> SRSKK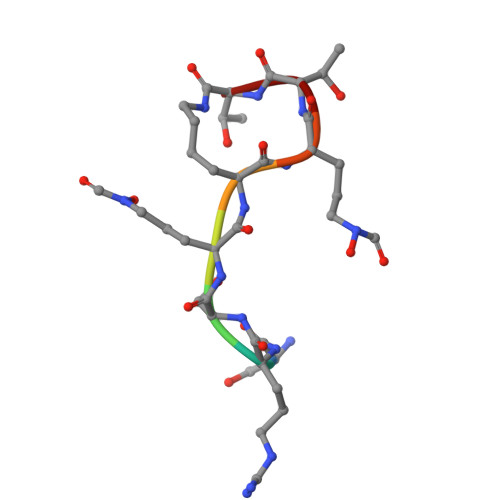KTT> GPLGSMSGIALSRLAQERKAWRKDHPFGFVAVPTKNPDGTMNLMNWECAIPGKKGTPWEGGLFKLRMLFKDDYPSSPPKCKFEPPLFHPNVYPSGTVCLSILEEDKDWRPAITIKQILLGIQELLNEPNIQDPAQAEAYTIYCQNRVEYEKRVRAQAKKFAPS;> GPLGSASKPEVTVRLNVHKVTVLTLQDKIVKEKFAMVAPDVQIEDGKGTILISSEEGETEANNHKKLSEFGIRNGSRLQADDFLQDYTLLINILHSEDLGKDVEFEVVG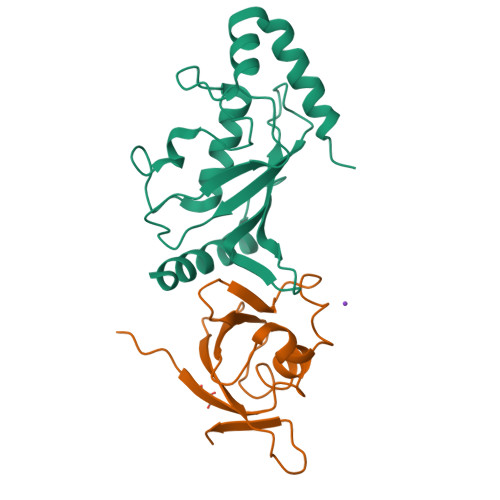DAPEKVGPKQAED> APAAVDWRARGAVTAVKDQGQCGSCWAFSAIGNVECQWFLAGHPLTNLSEQMLVSCDKTDSGCSGGLMNNAFEWIVQENNGAVYTEDSYPYASGEGISPPCTTSGHTVGATITGHVELPQDEAQIAAWLAVNGPVAVAVDASSWMTYTGGVMTSCVSEALDHGVLLVGYNDSAAVPYWIIKNSWTTQW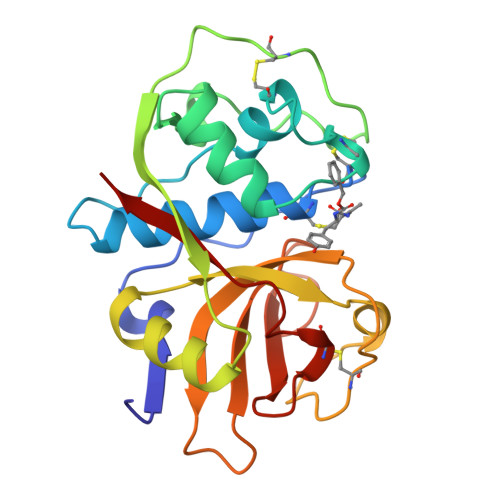GEEGYIRIAKGSNQCLVKEEASSAVVG One family of T3S effectors, the Cifs, re-program the host cell cycle causing arrest at the G2/M or the G1/S transition. In this study the crystal structures of Cif from P. luminescences (CifPl) and B. pseudomallei (CifBp) are presented. The structures reveal a head-and-tail domain arrangement, with the head-domain adopting an overall fold similar to papain-like cysteine proteases. The structure of the tail-domain of CifPl and CifBp presents an extensive surface area adjacent to the active site suggestive of a binding surface for interaction with a specific substrate.

MALDI-TOF analysis of purified CifPl is consistent with cleavage after residue Lys48 of the full-length sequence (assuming no cleavage at the C-terminus; Proteomics Facility, JIC, Norwich). This removes the unstructured region from the N-terminus that was identified bioinformatically, without the addition of exogenous protease. For CifPl, the N-terminal ∼48 residues are cleaved prior to crystallisation, therefore ∼2 residues expected to be in the crystallised protein but are not observed in the electron density. In CifPl the equivalent residues are Cys123, His181 and Gln200; in CifBp they are Cys90, His145 and Gln165. The active site cysteine is located at the N-terminus of 13 residue α-helix (α5) with the side chains of His181 and Gln200 arising from the β2 and β3-strands respectively. The thiol group of the putative catalytic cysteine is positioned 3.9 Å from the Nδ1 atom of His181 (CifPl numbering). The orientation of His181 is stabilised by a hydrogen bond from the Nε2 atom of this residue to the Oε1 atom of Gln200 (2.7 Å, CifPl numbering). The side chain of Asp202 (CifPl numbering) projects into a solvated pocket in Cifs and could be involved in either modulating the electrostatic properties of the active site or substrate binding. Mass fingerprinting analysis of CifPl localises the site of modification to the cysteine-containing peptide ‘IDESVSELGGLEMYQEMVGVNPYDPTEPVCGLSAQNIFK’, which shifts from 4261.5 Da (theoretical mass of 4260.8 Da) to 4472.8 Da (theoretical mass 4471.7 Da), an experimentally measured shift of 211.3 Da.

> KNSINTIKLIDDIIALHNDPKGNKLLWNDNWQDKIINRDLANIFEKIDESVSELGGLEMYQEMVGVNPYDPTEPVCGLSAQNIFKLMTEGEHAVDPVEMAQTGKIDGNEFAESVDQLSSAKNYVALVNDRRLGHMFLIDIPSNDQETVGYIYQSDLGQGALPPLKIADWLNSRGKDAVSLNKLKKLLSREFNLLSDDEKRALISETLDIHKDVSNVELDRIKRDRGVDIYLTEYDVNNFYENIETLKSKLSNYDKKLSKPK> SATTGARSASVGWAESLIGLHLGKVALITGGSAGIGGQIGRLLALSGARVMLAARDRHKLEQMQAMIQSELAEVGYTDVEDRVHIAPGCDVSSEAQLADLVERTLSAFGTVDYLINNAGIAGVEEMVIDMPVEGWRHTLFANLISNYSLMRKLAPLMKKQGSGYILNVSSYFGGEKDAAIPYPNRADYAVS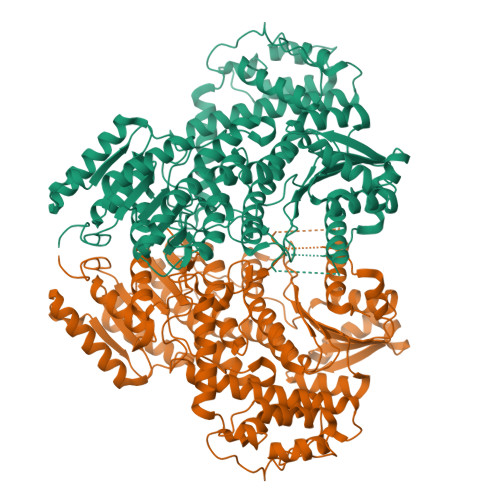KAGQRAMAEVFARFLGPEIQINAIAPGPVEGDQLRGTGERPGLFARRARLILENKRLNELHAALIAAARTDERSMHELVELLLPNDVAALEQNPAAPTALRELARRFRSEGDPAASSSSALLNRSIAAKLLARLHNGGYVLPADIFANLPNPPDPFFTRAQIDREARKVRDGIMGMLYLQRMPTEFDVAMATVYYLADRNVSGETFHPSGGLRYERTPTGGELFGLPSPERLAELVGSTVYLIGEHLTEHLNLLARAYLERYGARQVVMIVETETGAETMRRLLHDHVEAGRLMTIVAGDQIEAAIDQAITRYGRPGPVVCTPFRPLPTVPLVGRKDSDWSTVLSEAEFAELCEHQLTHHFRVARKIALSDGASLALVTPETTATSTTEQFALANFIKTTLHAFTATIGVESERTAQRILINQVDLTRRARAEEPRDPHERQQELERFIEAVLLVTAPLPPEADTRYAGRIHRGRAITV>DADLDKQVNTAGAWPIATGGYYSQHNSPLAQINKSNVKNVKAAWSFSTGVLNGHEGAPLVIGDMMYVHSAFPNNTYALNLNDPGKIVWQHKPKQDASTKAVMCCDVVDRGLAYGAGQIVKKQANGHLLALDAKTGKINWEVEVCDPKVGSTLTQAPFVAKDTVLMGCSGAELGVRGAVNAFDLKTGELKWRAFATGSDDSVRLAKDFNSANPHYGQFGLGTKTWEGDAWKIGGGTNWGWYAYDPKLNLFYYGSGNPAPWNETMRPGDNKWTMTIWGRDLDTGMAKWGYQKTPHDEWDFAGVNQMVLTDQPVNGKMTPLLSHIDRNGILYTLNRENGNLIVAEKVDPAVNVFKKVDLKTGTPVRDPEFATRMDHKGTNICPSAMGFHNQGVDSYDPESRTLYAGLNHICMDWEPFMLPYRAGQFFVGATLAMYPGPNGPTKKEMGQIRAFDLTTGKAKWTKWEKFAAWGGTLYTKGGLVWYATLDGYLKALDNKDGKELWNFKMPSGGIGSPMTYSFKGKQYIGSMYGVGGWPGVGLVFDLTDPSAGLGAVGAFRELQNHTQMGGGLMVFSL[2x];>YDGQNCKEPGNCWENKPGYPEKIAGSKYDPKHDPVELNKQEESIKAMDARNAK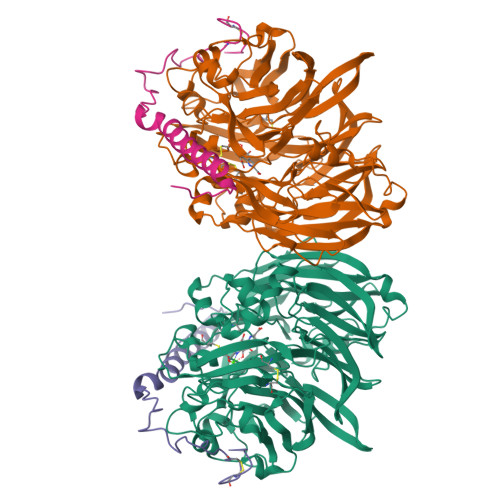RIANAKSSGNFVFDVK[2x]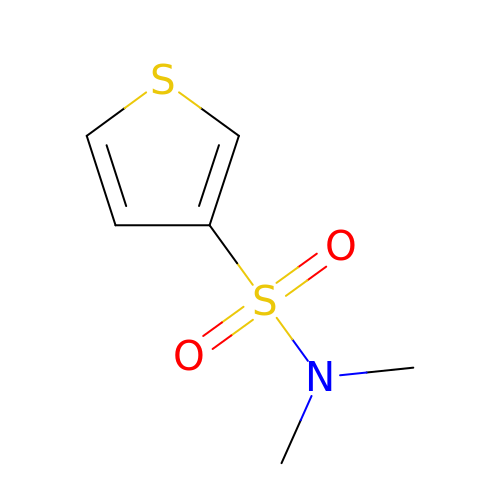N,N-dimethylthiophene-3-sulfonamide | C6 H9 N O2 S2 | ULWLGURUKSRLMX-UHFFFAOYSA-N>[10x]APADNAADARPVDVSVSIFINKIYGVNTLEQT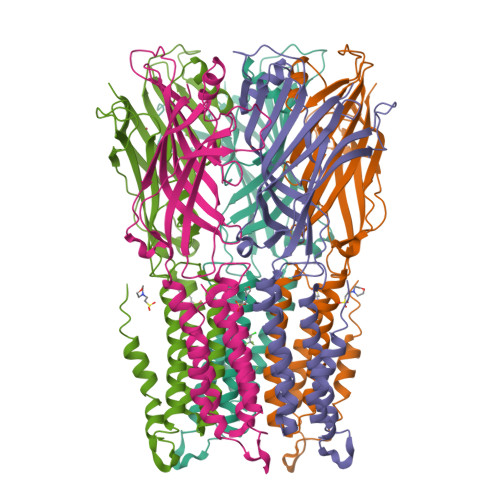YKVDGYIVAQWTGKPRKTPGDKPLIVENTQIERWINNGLWVPALEFINVVGSPDTGNKRLMLFPDGRVIYNARFLGSFSNDMDFRLFPFDRQQFVLELEPFSYNNQQLRFSDIQVYTENIDNEEIDEWWIRGKASTHISDIRYDHLSSVQPNQNEFSRITVRIDAVRNPSYYLWSFILPLGLIIAASWSVFWLESFSERLQTSFTLMLTVVAYAFYTSNILPRLPYTTVIDQMIIAGYGSIFAAILLIIFAHHRQANGVEDDLLIQRCRLAFPLGFLAIGCVLVIRGITL> DKATIPSESPFAAAEVADGAIVVDIAKMKYETPELHVKVGDTVTWINREAMPHNVHFVAGVLGEAALKGPMMKKEQAYSLTFTEAGTYDYHCT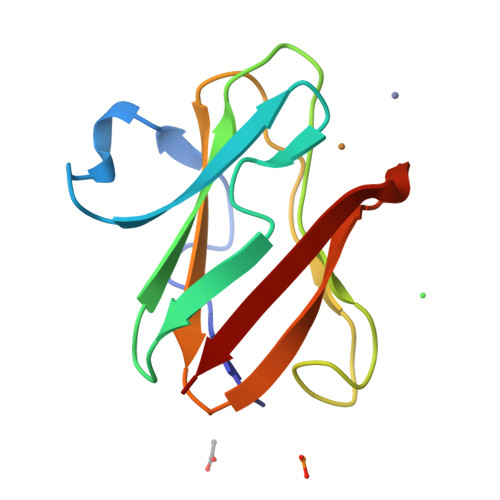PHPFLRGKVVVE>[9x]MAQILPIRFQEHLQLQNLGINPANIGFSTLTMESDKFICIREKVGEQAQVVIIDMNDPSNPIRRPISADSAIMNPASKVIALKAGKTLQIFNIEMKSKMKAHTMTDDVTFWKWISLNTVALVTDNAVYHWSMEGESQPVKMFDRHSSLAGCQIINYRTDAKQKWLLLTGISAQQNRVVGAMQLYSVDRKVSQPIEGHAASFAQFKMEGNAEESTLFCFAVRGQAGGKLHIIEVGTPPTGNQPFPKKAVDVFFPPEAQNDFPVAMQISEKHDVVFLITKYGYIHLYDLETGTCIYMNRISGETIFVTAPHEATAGIIGVNRKGQVLSVCVEEENIIPYITNVLQNPDLALRMAVRNNLAGAEELFARKFNALFAQGNYSEAAKVAANAPKGILRTPDTIRRFQSVPAQPGQTSPLLQYFGILLDQGQLNKYESLELCRPVLQQGRKQLLEKWLKEDKLECSEELGDLVKSVDPTLALSVYLRANVPNKVIQCFAETGQVQKIVLYAKKVGYTPDWIFLLRNVMRISPDQGQQFAQMLVQDEEPLADITQIVDVFMEYNLIQQCTAFLLDALKNNRPSEGPLQTRLLEMNLMHAPQVADAILGNQMFTHYDRAHI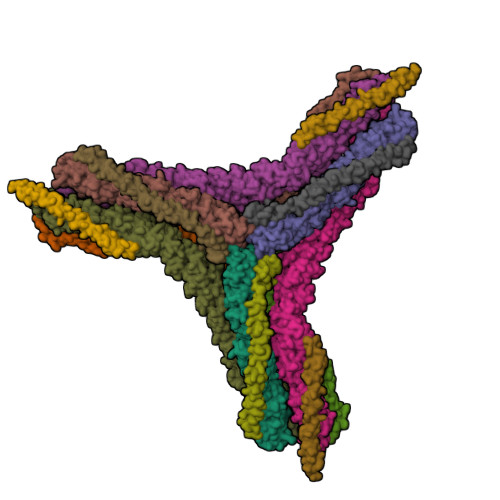AQLCEKAGLLQRALEHFTDLYDIKRAVVHTHLLNPEWLVNYFGSLSVEDSLECLRAMLSANIRQNLQICVQVASKYHEQLSTQSLIELFESFKSFEGLFYFLGSIVNFSQDPDVHFKYIQAACKTGQIKEVERICRESNCYDPERVKNFLKEAKLTDQLPLIIVCDRFDFVHDLVLYLYRNNLQKYIEIYVQKVNPSRLPVVIGGLLDVDCSEDVIKNLILVVRGQFSTDELVAEVEKRNRLKLLLPWLEARIHEGCEEPATHNALAKIYIDSNNNPERFLRENPYYDSRVVGKYCEKRDPHLACVAYERGQCDLELINVCNENSLFKSLSRYLVRRKDPELWGSVLLESNPYRRPLIDQVVQTALSETQDPEEVSVTVKAFMTADLPNELIELLEKIVLDNSVFSEHRNLQNLLILTAIKADRTRVMEYINRLDNYDAPDIANIAISNELFEEAFAIFRKFDVNTSAVQVLIEHIGNLDRAYEFAERCNEPAVWSQLAKAQLQKGMVKEAIDSYIKADDPSSYMEVVQAANTSGNWEELVKYLQMARKKARESYVETELIFALAKTNRLAELEEFINGPNNAHIQQVGDRCYDEKMYDAAKLLYNNVSNFGRLASTLVHLGEYQAAVDGARKANSTRTWKEVCFACVDGKEFRLAQMCGLHIVVHADELEELINYYQDRGYFEELITMLEAALGLERAHMGMFTELAILYSKFKPQKMREHLELFWSRVNIPKVLRAAEQAHLWAELVFLYDKYEEYDNAIITMMNHPTDAWKEGQFKDIITKVANVELYYRAIQFYLEFKPLLLNDLLMVLSPRLDHTRAVNYFSKVKQLPLVKPYLRSVQNHNNKSVNESLNNLFITEEDYQALRTSIDAYDNFDNISLAQRLEKHELIEFRRIAAYLFKGNNRWKQSVELCKKDSLYKDAMQYASESKDTELAEELLQWFLQEEKRECFGACLFTCYDLLRPDVVLETAWRHNIMDFAMPYFIQVMKEYLTKVDKLDASESLRKEEEQATETQPIVYGQPQLMLTAGPSVAVPPQAPFGYGYTAPPYGQPQPGFGYSM;>[6x]MADDFGFFSSSESGAPEVAEEDPAAAFLAQQESEIAGIENDEGFGAPAGSQAALAQPGPASGAGPEDMGTTVNGDVFQDANGPADGYAAIAQADRLTQEPESIRKWREEQRKRLQELDAASKVTEQEWREKAKKDLEEWNQRQSEQVEKNKINNRIADKAFYQQPDADIIGYVASEEAFVKESKEETPGTEWEKVAQLCDFNPKSSKQCKDVSRLRSVLMSLKQTPLSR>[6x]GPMSFLFGSRSSKTFKPKKNIPEGSHQYELLKHAEATLGSGNLRMAVMLPEGEDLNEWVAVNTVDFFNQINMLYGTITDFCTEESCPVMSAGPKYEYHWADGTNIKKPIKCSAPKYIDYLMTWVQDQLDDETLFPSKIGVPFPKNFMSVAKTILKRLFRVYAHIYHQHFDPVIQLQEEAHLNTSFKHFIFFVQEFNLIDRRELAPLQELIEKLTSKDR

To exert full kinase activity, MST1/2 and LATS1/2 requires coactivators, the scaffolding proteins Salvador homolog 1 (SAV1) and Mps One binder 1 (MOB1), respectively. Phosphorylated MOB1 protein is switched ON to increase the binding affinity to LATS1/2 and this binding accelerates auto-phosphorylation of the activation loop, A-loop (also referred to as activation segment or T-loop), of LATS1/2 kinases for full activation. The phosphorylation of MOB1 occurs at two threonine residues, Thr12 and Thr35, located at the N-terminal extension out of the C-terminal globular MOB core domain, and is required for binding to LATS/NDR kinases. Here we report the results of structural and biochemical studies of full-length mouse MOB1B in the autoinhibited form and that of the MOB core domain bound to the NTR region of LATS1 (hereafter referred to as the MOB1B-LATS1 complex).

However, we successfully purified full-length MOB1B by low-temperature expression (see experimental procedures) and quick purification without degradation, and determined the three-dimensional structure at 2.2 Å resolution. The overall structure adopts a globular shape comprising the MOB core domain made of nine α-helices (H1-H9) with the N-terminal extension, which forms a β-strand (the SN strand, residues 5-9) at the N-terminal segment of FLFGSRSS (residues 3-10) and a newly formed 4-turn α-helix (residues 24-38, hereafter referred to as the Switch helix), whereas the 10-residue linker between the SN strand and the Switvch helix were poorly defined on the current map. Notablly, the SN strand forms a β-sheet with the S2 strand (residues 95-98). One zinc ion is coordinated by two cysteine (Cys79 and Cys84) and two histidine (His161 and His166) residues and linked to the H3-S1 loop and the C-terminal part of the H5 helix as found in the structures of other MOB proteins. The Switch helix-binding site on the MOB core domain is formed by helices H1, H2 and H7 and the H4-H5 loop, and is characterized by a conserved cluster of negative charges with nonpolar patches. This site is overlapped with the LATS1 binding surface found in the structures of the pMOB1A-LATS1 complex34, the Mob2p-Cbk1p complex36 and our MOB1B-LATS1 complex, which are described below in detail, suggesting that the autoinhibition is caused by Switch helix binding, which structurally blocks LATS/NDR binding. Positively-charged His24 forms salt bridges with Glu51 and Glu55 and bifurcated hydrogen bonds to Glu51 to lock the Switch helix onto the MOB core domain. The phosphorylation residue of Switch helix (Thr35) is located at the edge of the interface with the MOB core domain and forms two hydrogen bonds to the helix main chains. Therefore, once phosphorylation occurs, phosphorylated Thr35 structurally inhibits binding of the Switch helix to the MOB core domain, which is consistent with previous reports that showed a critical role of Thr35 phosphorylation in LATS2 activation.> ADTVTLPFANGERPLVMYPGKRPLIGLTARPPQLETPFSVFDEGLITP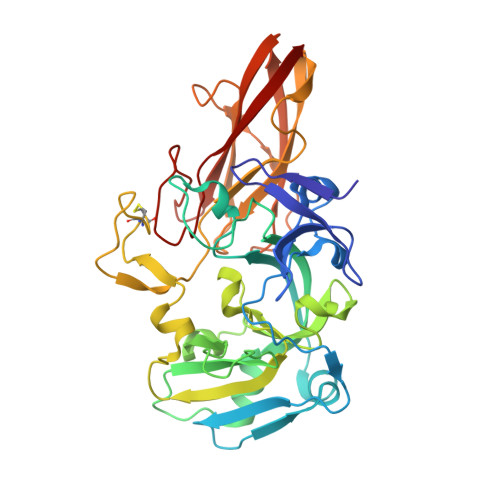NDAFFVRYHLAGIPLEIDPDAFRLEIKGKVGTPLSLSLQDLKNDFPASEVVAVNQCSGNSRGFVEPRVGGGQLANGAMGNARWRGVPLKAVLEKAGVQAGAKQVTFGGLDGPVIPETPDFVKALSIDHATDGEVMLAYSMNGADLPWLNGYPLRLVVPGYYGTYWVKHLNEITVIDKEFDGFWMKTAYRIPDNACACTEPGKAPTATIPINRFDVRSFITNVENGASVKAGEVPLRGIAFDGGYGITQVSVSADAGKSWTNATLDPGLGKYSFRGWKAVLPLTKGDHVLMCRATNARGETQPMQATWNPAGYMRNVVEATRVIAA> MSGSENEKLVEKVLEATRRIAREEAVKYKDAFLRAYRARDGAGLRRVITGLFSKVDSRLYKEVLTDVPTIVALQRRA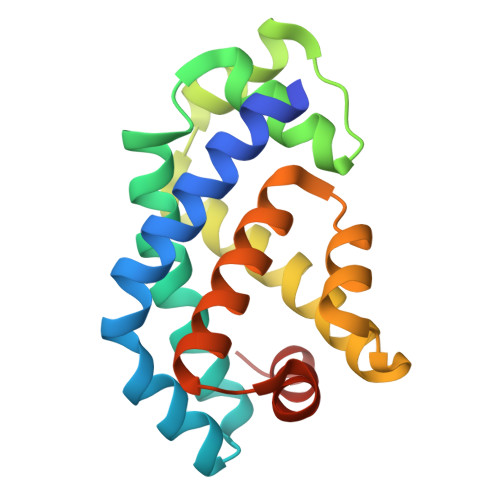GVDITPEQAQEILDNYDNEKHTAAVMDETFALLARAAATQASYEELLAAAPSGSVILALEVLRVLLEINNLSWREVLPLLALAAASGSG> QAGDTLNDVIQDPTRRNKLINDNNLLKGIIMGRDGPVPSSRELIVRPDTLRAIINNRATIETTTMEAEFTETLMESNYNSASVKVSAPFITANSEYSESSSFKNTETEKSMYTSSRYLFPQGRIDFTTPDSGFDDVIKLSPQFTSGVQAALAKATGTEKREALQNLFQEYGHVFRTKVHIGGVLSAHTMETFSRSENETEVKQDVKAGLEGAVKGWGGGATAGHGNTQGTITTSQNRKLNVKYIVNGGDYTKIQNTEEWVASTNQSEHWRVIEVTEVTAVADLLPQPIRGQVKDLLKPLLGKWVDVEKVPGLESLPVSVYRPKGAIPA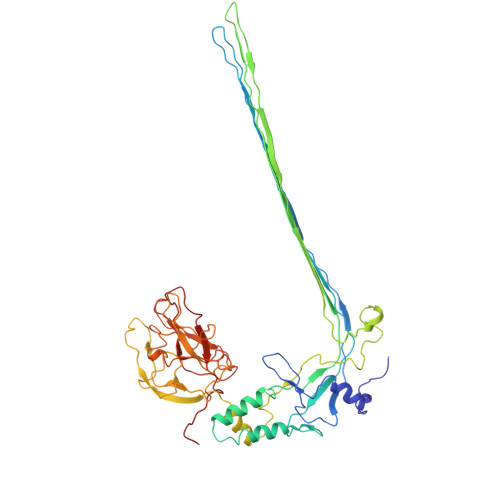GWFWLGDTADASKALLVKPTLPARSGRNPALTSLHQGSGMTEQPFVDLPQYQYLSTYFGSFAHDTPPGSTLRGLRPDHVLPGRYEMHGDTISTAVYVTRPVDVPFPEDECFDLKSLVRVKLPGSGNPPKPRSALKKSMVLFDSGEK> 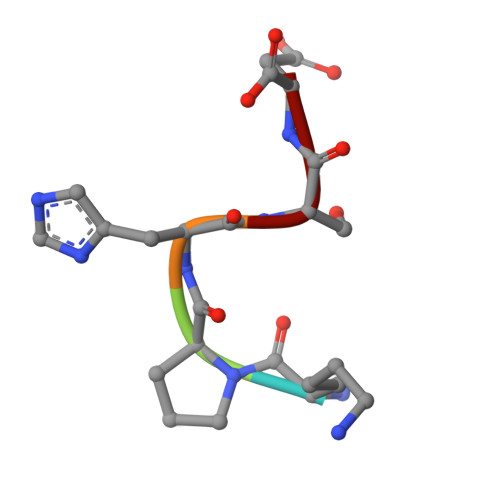KPHSD>PMFIVNTNVPRASVPDGFLSELTQQLAQATGKPPQYIAVHVVPDQLMAFGGSSEPCALC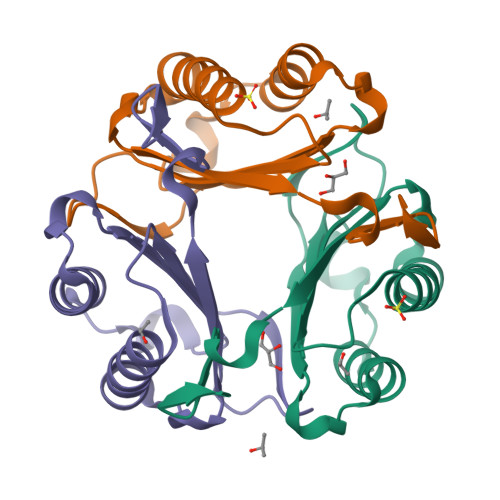SLYSIGKIGGAQNRSYSKLLCGLLAERLRISPDRVYINYYDMNAANVGWNNSTFA[3x]> S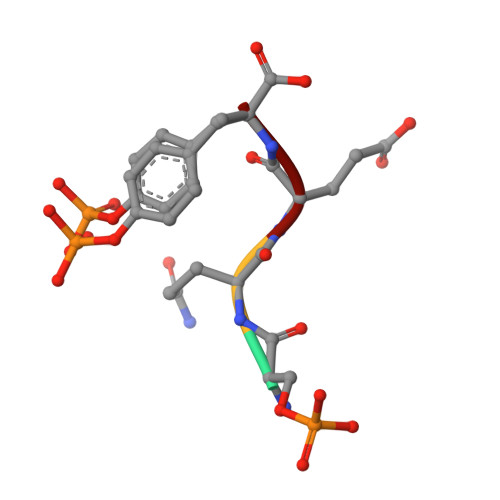QEY>AQESPAFIDPASWNTPFNGIAQVACHNCYEKQYANTFSSVLDSVRTLELDFWDQRDAVSGGS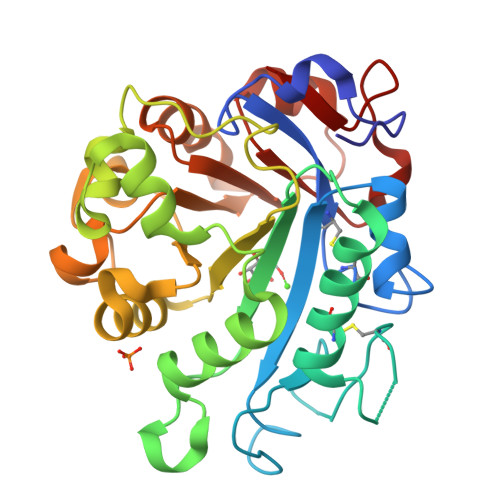PHHWFVRHNPGTLFQSGNDNNCTGDGTGKNDLEACLNDVKNWSDKHPGHFPITLILDKKQGWSKESSGRTPKDFDELVARVFQGKLFTPQDLATHIGSGAGALQGNLKGKSWPTANDLQGKVLLVLNHSENQKLSQYAEARTSKAKVFISPVTNGQNDISGKVSGMSSQSSGYVAMNNMGKGDKSWAKQAFAYSHIGRVWGDDEVSFAQHINQKINLSAYYRFAAQSAGGYRIRPF[4x]> LDGFKDSFD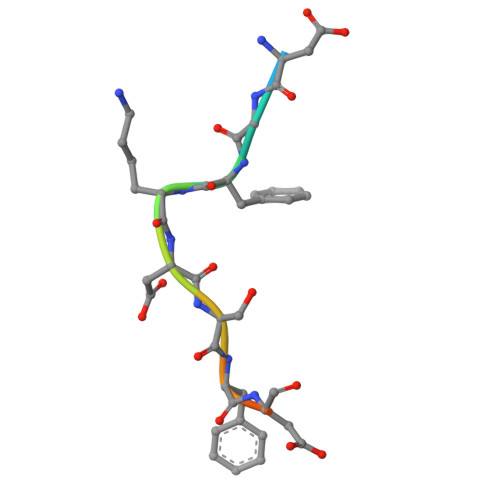LQG> MIVLFVDFDYFAAQVEEVLNPSLKGKPVVVCVFSGRFEDSGAVATANYEARKFGVKAGIPIVEAKKILPNAVYLPMRKEVYQQVSSRIMNLLREYSEKIEIASIDE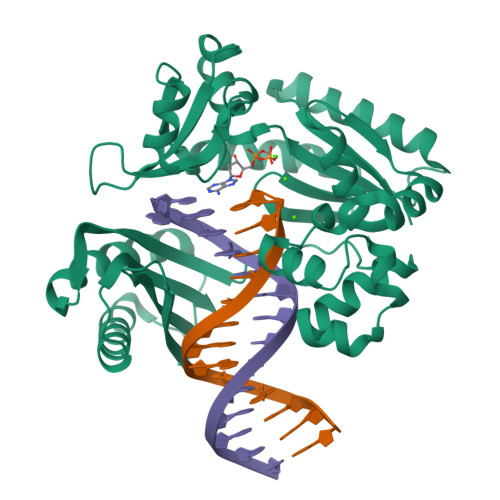AYLDISDKVRDYREAYNLGLEIKNKILEKEKITVTVGISKNKVFAKIAADMAKPNGIKVIDDEEVKRLIRELDIADVPGIGNITAEKLKKLGINKLVDTLSIEFDKLKGMIGEAKAKYLISLARDEYNEPIRTRVRKSIGRIVTMKRNSRNLEEIKPYLFRAIEESYYKLDKRIPKAIHVVAVTEDLDIVSRGRTFPHGISKETAYSESVKLLQKILEEDERKIRRIGVRFSKFI>[5x]MGAAAAEADRTLFVGNLETKVTEELLFELFH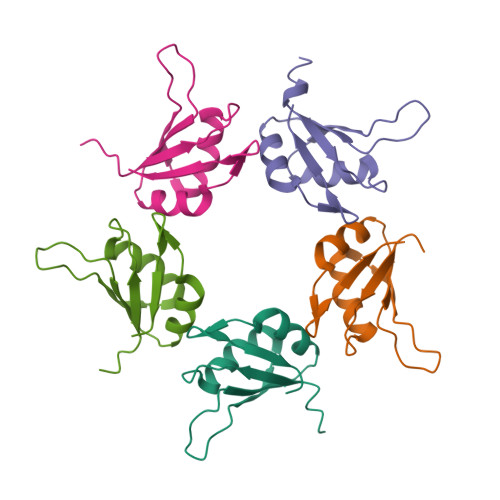QAGPVIKVKIPKDKDGKPKQFAFVNFKHEVSVPYAMNLLNGIKLYGRPIKIQFRSGSSHA> KTTSSALKGAIQLGITHSVGSLSQKPERDVLMQDFEVVESIFFPSQGSSSTPGHHHGDFKFKTYAPIAFRYFREMFGIRPDDYLYSLCNEPLIELSNPGASGSLFYVSSDDEFIIKTVQHKE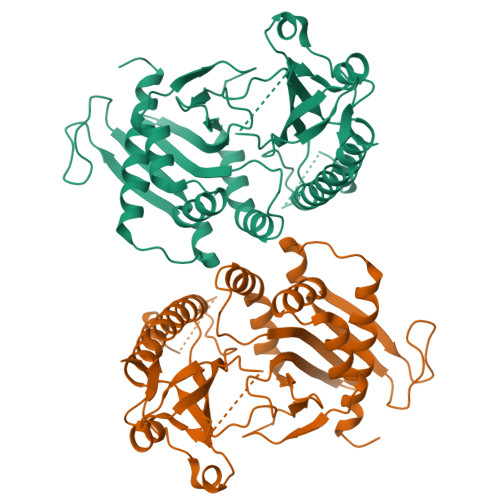AEFLQTLLPGYFMNLNQNMRTLLPKFYGLYCVQADGKNIRIVVMNNLLPRAVPMHLKFDLKGSTYKRRASPKERSKGVPTYKDLDFMQDMPEGILLENDHYTALSRTMQRDCRVLQSFKIMDYSLLVGIHILHRAGEEASTAVPDTQKKGQGQKPLYCTAIESIQGESKSKTSPQPYESMGGIPAFNSKGERLLVFIGIIDILQSYRLVKKLEHSWKALLHDGDTVSVHRPSFYADRFQKFMCSTVFRKS> MAHHHHHHMLHNTFFICETNQIMNEIEKAKGIILNRNMNDIWSALLIEVKKSNLIIKSTDRNIFFESTISIVSETDFKVLINASNFYDAVKAFNFYKKIKIVFNENNSKLEIMGELNDEKEEYEDHLKEPTFSYEEIENYNYDMVNEDYTFGIEIKQKSFKKVINRIAFSAHLDESKNVLNGVYFSKDEDSKLLLVSTNGHR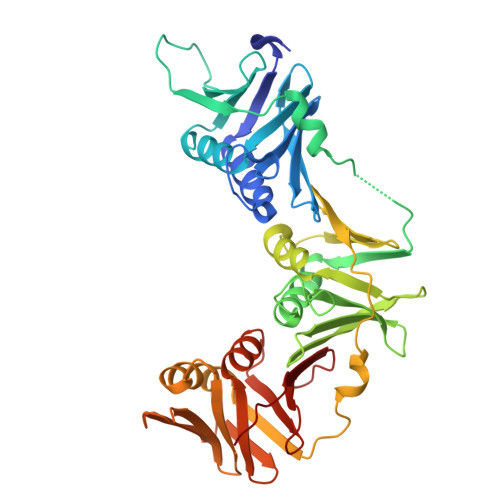MSICKTEVIVEEDVNFIVPVKIFNFLKHLMSGEGMVKIKFSDKKFYVEFDNYKIACSLINGNYPDYKSIIPKEQKNKSLVSLGILKDRLARVNLYVDKSRKLVLTFSELQLKLLGEDLITGRKGEFFIKDPNYLYDGADEVMAINISYFVEAISVFETSKIEIQFNSGNVLKLSEPENFNFTHLIMPMSLG> EDKRAKVTSAMQTMLFTMLRKLDNDALNNIINNARDGCVPLNIIPLTTAAKLMVVIPDYNTYKNTCDGTTFTYASALWEIQQVVDADSKIVQLSEISMD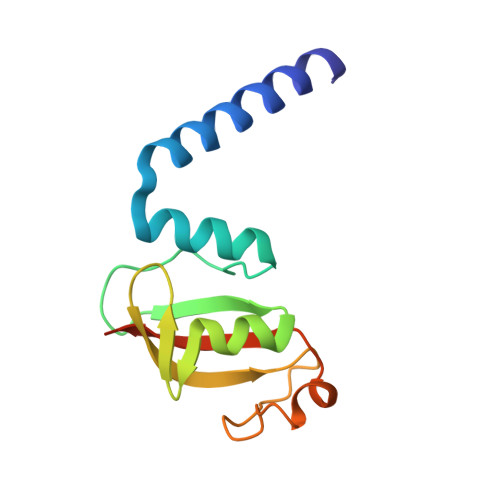NSPNLAWPLIVTALRANSAVKLQ>[6x]GEPRTRAEARPWVDEDLKDSSDLHQAEEDADEWQESEENVEHIPFSHNHYPEKEMVKRSQEF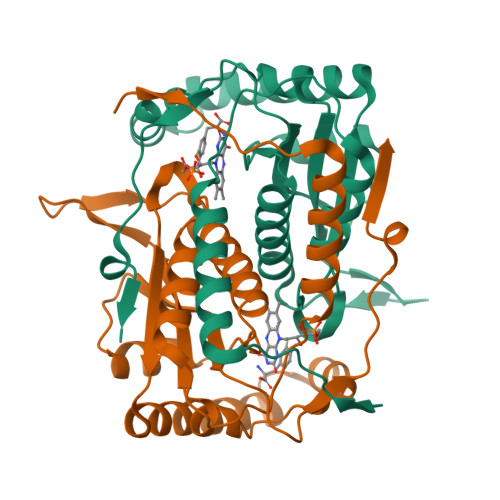YELLNKRRSVRFISNEQVPMEVIDNVIRTAGTAPSGAHTEPWTFVVVKDPDVKHKIRKIIEEEEEINYMKRMGHRWVTDLKKLRTNWIKEYLDTAPILILIFKQVHGFAANGKKKVHYYNEISVSIACGILLAALQNAGLVTVTTAPLNCGPRLRVLLGRPAHEKLLMLLPVGYPSKEATVPDLKRKPLDQIMVTVHHHHHH>[3x]MASIRLADLAQQLDAELHGDGDIVITGVASMQSAQTGHITFMVNPKYREHLGLCQASAVVMTQDDLPFAKSAALVVKNPYLTYARMAQILDTTPQPAQNIAPSAVIDATAKLGNNVSIGANAVIESGVELGDNVIIGAGCFVGKNSKIGAGSRLWANVTIYHEIQIGQNCLIQSGTVVGADGFGYANDRGNWVKIPQIGRVIIGDRVEIGACTTIDRGALDDTIIGNGVIIDNQCQIAHNV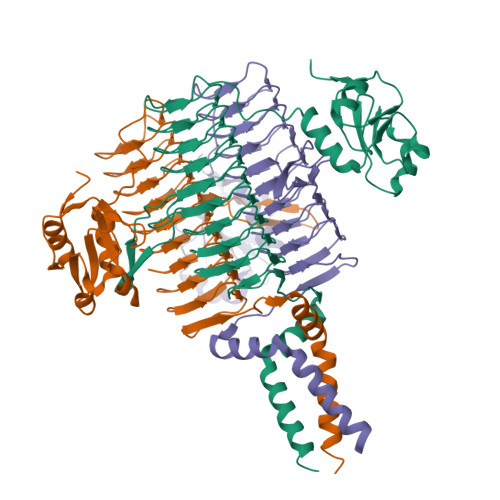VIGDNTAVAGGVIMAGSLKIGRYCMIGGASVINGHMEICDKVTVTGMGMVMRPITEPGVYSSGIPLQPNKVWRKTAALVMNIDDMSKRLKSLERKVNQQD> MSEGFSSSSIQELYQSLKEITNNADVELFEDRITKLDFESTDEPKHANDIIKDRFLRPSNALPWSLLDMVQDVPHTSSPEDCSGKLDYKELLKVPDPINRTSYQFKRTGLEGKISGYKEEVDLKEVANANASNSLSITRSINHNQNSVRGSTAQLPFTPGGIPMKSVKTDSEQNGSSTMANATKLLHKDGQGLFDIPEGMNRGIKPMDSPAENEDQNGQFKELKQLNEIDNELDIRIEANEAKLKEEEKSAKSISEEIMEEATEETTADNADDAEIDELLPIGIDFGRTKPVSKSVPVKKEWAHVVDLNHKIENFDELIPNPARSWPFELDTFQKEAVYHLEQGDSVFVAAHTSAGKTVVAEYAIAMAHRNMTKTIYTSPIKALSNQKFRDFKETFDDVNIGLITGDVQINPDANCLIMTTEILRSMLYRGADLIRDVEFVIFDEVHYVNDQDRGVVWEEVIIMLPQHVKFILLSATVPNTYEFANWIGRTKQKNIYVISTPKRPVPLEINIWAKKELIPVINQNSEFLEANFRKHKEILNGESAKGAPSKTDNGRGGSTARGGRGGSNTRDGRGGRGNSTRGGANRGGSRGAGAIGSNKRKFFTQDGPSKKTWPEIVNYLRKRELLPMVVFVFSKKRCEEYADWLEGINFCNNKEKSQIHMFIEKSITRLKKEDRDLPQILKTRSLLERGIAVHHGGLLPIVKELIEILFSKGFIKVLFATETFAMGLNLPTRTVIFSSIRKHDGNGLRELTPGEFTQMAGRAGRRGLDSTGTVIVMAYNSPLSIATFKEVTMGVPTRLQSQFRLTYNMILNLLRIEALRVEEMIKYSFSENAKETLQPEHEKQIKVLQEELQTIEYKSCEICDNDIEKFLELMLAYKEATVNLMQEMVKSPSILHILKEGRLVAFRDPNDCLKLGFVFKVSLKDAVCVIMTFTKPYKLPNGEPNHLIYFPKADGYRRRNFPKFQKTDFYMEEVPVTAIEVITKRKFAAPLGKVIKKDVAALNEFNAETNNILDGKTLKEAINIEKQGLKIHQILLDRTNIRDEIFKLKSIKCPNLSQHIVPKFKAHVIKKKIEELYHLMSDQNLSLLPDYEKRLAVLKDTEFIDQNHNVLLKGRVACEINSGYELVLTELILDNFLGSFEPEEIVALLSVFVYEGKTREEEPPIVTPRLAKGKQRIEEIYKKMLCVFNTHQIPLTQDEAEFLDRKRFAMMNVVYEWARGLSFKEIMEMSPEAEGTVVRVITWLDEICREVKTASIIIGNSTLHMKMSRAQELIKRDIVFAASLYL;> GPDSMSDIKQLLKEAKQELTNRDYEETIEISEKVLKLDPDNYFAHIFLGKALSSLPASNNVSSNRNLERATNHYVSAAKLVPDNLLAWKGLFLLFRTTEVVPDILSYDEYFDLCGQYADALLKQEQSQVELINDIKLLKKTHPDCQKAFYQHLKPGSLMAETIGRHLSTPQDALLNLIKILSNIETTEIGKTLSQNRLKLKASDPDYQIKLNSFSWEIIKNSEIDQLYNQLVNILADDQKRSEIENQWLEYRIKVLKSMPLDVKKDFFTKVKEMVEDMVLVNHQSLLAWQKYFEWTDYEDLDNMDAPLIIKYFKKFPKDPLAMILYSWLSSKLSKYDIKSLESANKPPEGHKKTEKETDIKDVDETNEDEVKDRVEDEVKDRVEDEVKDQDEEAKEDEEEDLDDIEIGLLEEEVVTVLTENIVKCKNNILAHRILCQYYLLTKEYEAALPYIKNGISLIAYNIKDLGVHLPLTKREFSLDLATVYTYVDAPKDHNAALKLYDNILSGDFSNIQAKMGKGIIFIERKNWKDAMTLLTQVHEQSPNNLEVLSELSWSKAHMGYMDEALAGLDTVIKGIKGMDLRSIDFRALNLWRQAKVYIMKHASINDAK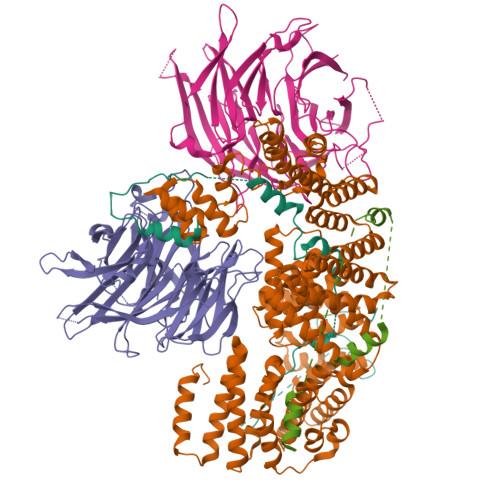QENVKCAFKLLIQSIKILDTFAPGFSTLGDIYCHYYKDHLRAFKCYFKAFDLDAGDYTAAKYITETYASKPNWQAASSIASRLIKGEKAKAELRSNNWPFRVVGIAHLEKQEESDSIEWFQSALRVDPNDVESWVGLGQAYHACGRIEASIKVFDKAIQLRPSHTFAQYFKAISLCDVGEYLESLDILEKVCQEAATEESFQIGLVEVLMRCSLDLYSQGFLLKSVSIAKDTIERIKIIISELKCENQQVWIYLSQVLRLFIWIESKVDTLPVESLVSIFENSQFSGSEEIDSVDNIKIDTLLDSTTDDNVSIACKFLILASKYSVSDQKFTDIAGTVRASYWYNIGISELTAFITLKEPQYRDAAIFAFKKSIQLQSNTSETWIGLGIATMDINFRVSQHCFIKATALEPKATNTWFNLAMLGLKKKDTEFAQQVLNKLQSLAPQDSSPWLGMALILEEQGDIIGSSKLFAHSFILSNGRSKAAQFMYAKNVLENHINNGDDERDIETVEKLTTASIALEQFFKKSPDSQFALQCALLTLERLHHYENANELANRLIGILEKKFEKTQDERELFNFAIIKGQFARIHLGLGNFELSIENADLSQGIISESSDEKSMKTKISNHICLGLSYFFLNDFDQTLNQFQELLSISKDSKHLVVLIAKVLYDVGESDTKEIALQELTEYIATSGADLLVTLTIAAMSILDDKREDLSIILEELKALPLSKQIIDKHKDAPYLIEEITKRLYRNDTGKQVWQRSAYFFPNNLKVWERLDKNIQRRIASNGQNKVTAEEMSKLYCESKNLRSIQRGMFLCPWNVTAVKALNECF;>MSKVFIATANAGKAHDADIFSVSACNSFTVSCSGDGYLKVWDNKLLDNENPKDKSYSHFVHKSGLHHVDVLQAIERDAFELCLVATTSFSGDLLFYRITREDETKKVIFEKLDLLDSDMKKHSFWALKWGASNDRLLSHRLVATDVKGTTYIWKFHPFADESNSLTLNWSPTLELQGTVESPMTPSQFATSVDISERGLIATGFNNGTVQISELSTLRPLYNFESQHSMINNSNSIRSVKFSPQGSLLAIAHDSNSFGCITLYETEFGERIGSLSVPTHSSQASLGEFAHSSWVMSLSFNDSGETLCSAGWDGKLRFWDVKTKERITTLNMHCDDIEIEEDILAVDEHGDSLAEPGVFDVKFLKKGWRSGMGADLNESLCCVCLDRSIRWFREAGGK[2x];> GPDSMSLLEQLARKRIEKSKGLLSADQSHSTSKSASLLERLHKNRETKDNNAETKRKDLKTLLAKDKVKRSDFTPNQHSVSLSLKLSALKKSNSDLEKQGKSVTLDSKENELPTKRKSPDDKLNLEESWKAIKEMNHYCFLKNDPCINQTDDFAFTNFIIKDKKNSLSTSIPLSSQNSSFLSLKKHNNELLGIFVPCNLPKTTRKVAIENFNRPSPDDIIQSAQLNAFNEKLENLNIKSAGSWSHPQFEK>[2x]MHHHHHHSNSAETDVLIVGAGPAGAMSATLLASLGIRSLMINRWRSTSPGPRSHIINQRTMEILRDIGLEESAKSLAVPKEYMGEHVYATSLAG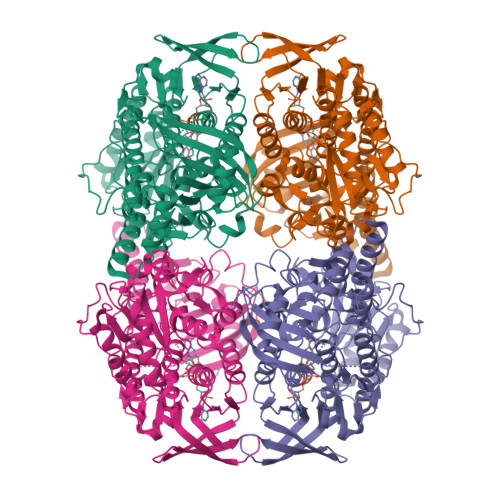EEFGRIPAWASHPQAHAEHELASPSRYCDLPQLYFEPMVVSEAALRGADVRFLTEYLGHVEDQDGVTARLLDHVSGAEYEVRAKYIIGADGAHSLVAQNAGLPFEGQMGIGDSGSINIEFSADLSSLCEHRKGDMYYMFRAGSGINGVGVAALRMIRPWNKWICVWGYEKSKGTPEITKEEAKKIIHEIIGTDEIPVEVGPISTWTINQQYAVRNTSGRVFCMGDAVHRHTPMGGLGLNTSVQDAYNLAWKLALVLKGTAAPTLLDSYDAERSPVAKQIVERAFKSLSTFPPVFEALSLPPAPTESEMAEALVRLKDASEEGAKRRAALRKAMDATIIGLGGGHGVELNQRYVSRAVFPDGTPDPGFVRDQEFFYQASTRPGAHLPHVWLTENQRRISTLDLCGKGRFTLLTGLSGAAWKHEAEQVSQSLGIELKVCVIGPGQEFVDTYGEYAKISEIGESGALLVRPDMFIAFRAKDASREGLEQLNVAVKSILGRA> GDLAAAKPALDAALEALNSIKDGDIKNLKALKKPPQIITRIFDCVLVLRMLPVTKAEYTDEKGRMVQVGNYPEAQKMMNQMSFLQDLK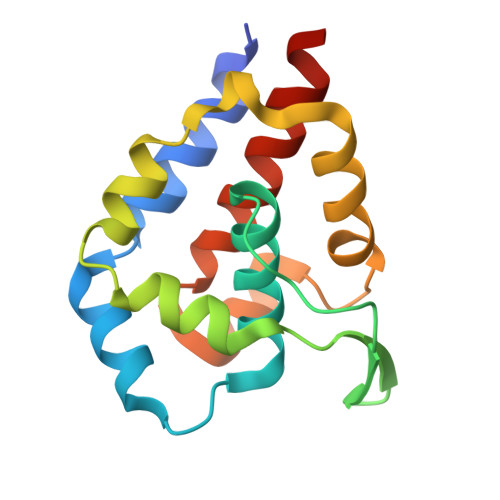DFAKEQINDETVELLEPYFMSEDFTFENAQKASGNVAGLCNWAESMAKYHNVAKVVE>[6x]MESNNGIILRVAEANSTDPGMSRVRLDESSRRLLDAEIGDVVEIEKVRKTVGRVYRARPEDENKGIVRIDSVMRNNCGASIGDKVKVRKVRTEIAKKVTLAPIIRKDQRLKFGEGIEEYVQRALIRRPMLEQDNISVPGLTLAGQTGLLFKVVKTLPSKVPVEIGEETKIEIREEPASEVLEEVSRISYEDIGGLSEQLGKIREMIELPLKHPELFERLGITPPKGVILYGPPGTGKTLIARAVANESGANFLSINGPEIMSKYYGQSEQKLREIFSKAEETAPSIIFIDEIDSIAPKREEVQGEVERRVVAQLLTLMDGMKERGHVIVIGATNRIDAIDPALRRPGRFDREIEIGVPDRNGRKEILMIHTRNMPLGMSEEEKNKFLEEMADYTYGFVGADLAALVRESAMNALRRYLPE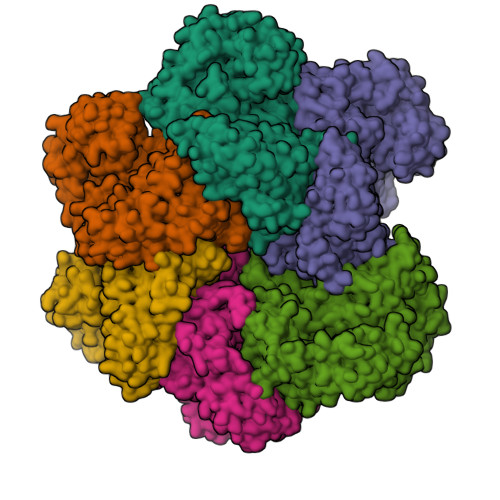IDLDKPIPTEILEKMVVTEDDFKNALKSIEPSSLREVMVEVPNVHWDDIGGLEDVKREIKETVELPLLKPDVFKRLGIRPSKGFLLYGPPGVGKTLLAKAVATESNANFISIKGPEVLSKWVGESEKAIREIFKKAKQVAPAIVFLDEIDSIAPRRGTTSDSGVTERIVNQLLTSLDGIEVMNGVVVIGATNRPDIMDPALLRAGRFDKLIYIPPPDKEARLSILKVHTKNMPLAPDVDLNDIAQRTEGYVGADLENLCREAGMNAYRENPDATSVSQKNFLDALKTIRPSVDEEVIKFYRTLSET> MALSMTGGQQMGRGSMSRDPLPFFPPLYLGGPEIT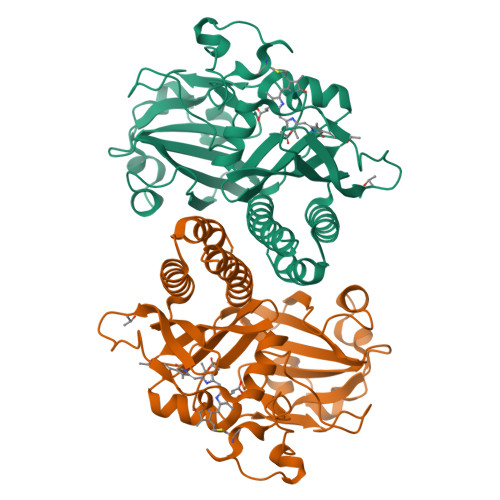TENCEREPIHIPGSIQPHGALLTADGHSGEVLQMSLNAATFLGQEPTVLRGQTLAALLPEQWPALQAALPPGCPDALQYRATLDWPAAGHLSLTVHRVGELLILEFEPTEAWDSTGPHALRNAMFALESAPNLRALAEVATQTVRELTGFDRVMLYKFAPDATGEVIAEARREGLHAFLGHRFPASAIPAQARALYTRHLLRLTADTRAAAVPLDPVLNPQTNAPTPLGGAVLRATSPMHMQYLRNMGVGSSLSVSVVVGGQLWGLIACHHQTPYVLPPDLRTTLESLGRLLSLQVQVKEAHHHHHH9-cyclopentyl-9H-purin-6-amine | 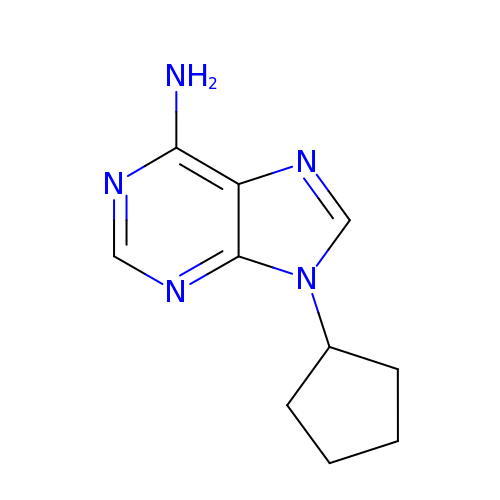C10 H13 N5 | KTJWHJNBTXITCB-UHFFFAOYSA-N2-[(4S)-6-(4-chlorophenyl)-8-methoxy-1-methyl-4H-[1,2,4]triazolo[4,3-a][1,4]benzodiazepin-4-yl]-N-ethylacetamide 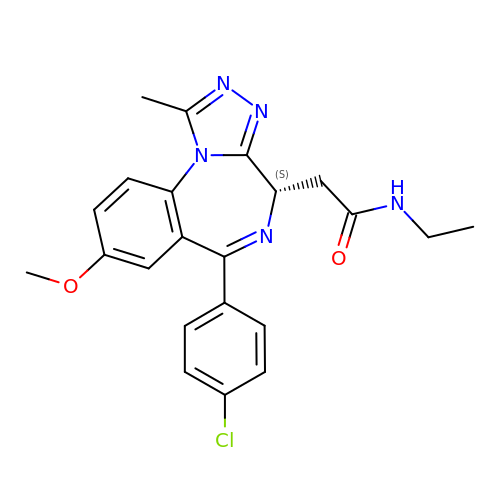| C22 H22 Cl N5 O2 | AAAQFGUYHFJNHI-SFHVURJKSA-N>MASQNRDPAATSVAAARKGAEPSGGAARGPVGKRLQQELMTLMMSGDKGISAFPESDNLFKWVGTIHGAAGTVYEDLRYKLSLEFPSGYPYNAPTVKFLTPCYHPNVDTQGNISLDILKEKWSALYDVRTILLSIQSLLGEPNIDSPLNTHAAELWK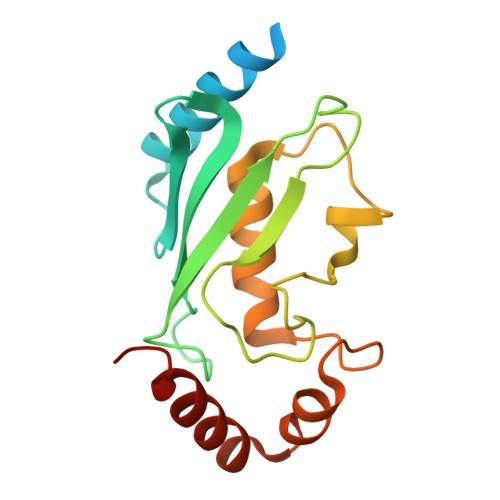NPTAFKKYLQETYSKQVTSQEP[2x]>[4x]MAGAVGRPRRSAPRRAGKNPREEILDASAELFTHQGFATTSTHQIA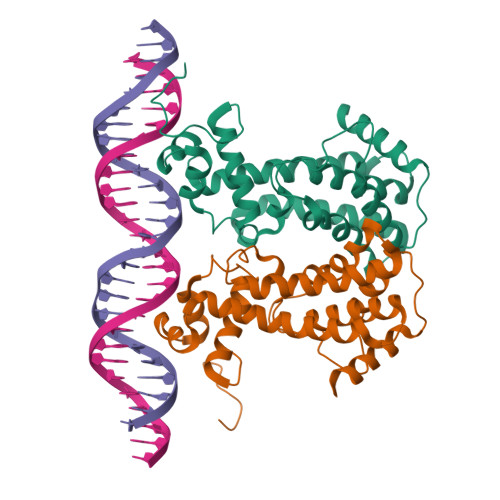DAVGIRQASLYYHFPSKTEIFLTLLKSTVEPSTVLAEDLSILDAGPEMRLWAIVASEVRLLLSTKWNVGRLYQLPIVGSEEFAEYHSQREALTNIFRDLATEIVGDDPRAELPFHITMSVIEMRRNDGKIPSPLSADSLPETAIMLADASLAVLGASLPADRVEKTLELIKQADAKLEHHHHHH>AMAQREIRLVDNEYPSPSMTHPPIPLSDIALTGIFEISKILTSPARLEITLANVVNLLQSFLQMRNGVVSLLADDGVPDITVGVGWNEGSDNRYRARLPQKAIDQIVATAVPLVADNVSAHPMFTAADAMALGATDEIRVSFIGVPIRIDSRV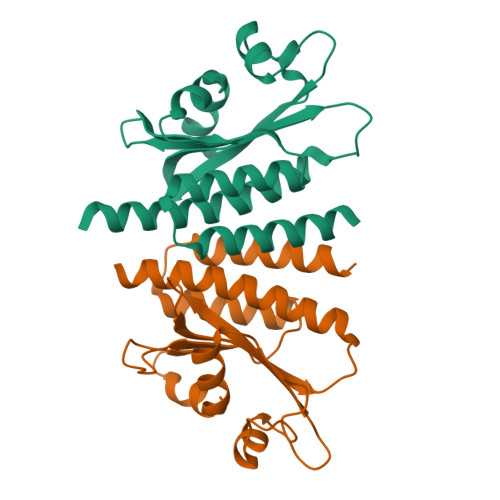VGTLSIDRVRDGRSHFRMDADVRFLTMVANLIGQTVKLHRVVARDRERLMAESHRL[2x]Transcription activator-like (TAL) effectors specifically bind to double stranded (ds) DNA through a central domain of tandem repeats. Each TAL effector (TALE) repeat comprises 33–35 amino acids and recognizes one specific DNA base through a highly variable residue at a fixed position in the repeat. The crystal structures of TAL effector (TALE) proteins bound to their respective target DNAs have revealed that the residue at position 13 is the only one directly involved in DNA base recognition, whereas the 12th residue stabilizes the proper loop conformation. dHax3, an engineered TALE protein, proved to be a useful scaffold for structural characterizations. We then present fifteen crystal structures of engineered dHax3 variants in complex with target DNA molecules, which elucidate the structural basis for the recognition of bases adenine (A) and guanine (G) by reported or uncharacterized TALE codes.

When the natural TALE codes were discovered, no code was found highly specific for base G. In light of the structures of the DNA-binding zinc finger proteins where positive charged amino acids such as Arg, His, Lys play a critical role in the coordination of base G, we made a dHax3 variant with an Arg34, His34, Lys34 in the 7th repeat. We then attempted to co-crystallize these proteins with a modified dHax3 box element whose 7th base is changed from A to G. Four complex structures were determined at high resolutions.

>[2x]MQWSGARALEALLTVAGELRGPPLQLDTGQLLKIAKRGGVTAVEAVHAWRNALTGAPLNLTPEQVVAIASHDGGKQALETVQRLLPVLCQAHGLTPQQVVAIASHDGGKQALETVQRLLPVLCQAHGLTPEQVVAIASHDGGKQALETVQALLPVLCQAHGLTPEQVVAIASNGGGKQALETVQRLLPVLCQAHGLTPQQVVAIASNGGGKQALETVQRLLPVLCQAHGLTPQQVVAIASNGGGKQALETVQRLLPVLCQAHGLTPQQVVAIASNKGGKQALETVQRLLPVLCQAHGLTPQQVVAIASNGGGKQALETVQRLLPVLCQAHGLTPQQVVAIASHDGGKQALETVQRLLPVLCQAHGLTPEQVVAIASNGGGKQALETVQRLLPVLCQAHGLTPEQVVAIASHDGGKQALETVQRLLPVLCQAHGLTPQQVVAIASNGGGRPALESIVAQLSRPDPALAALTNDHLVALACLGGRPALDAVKKLEHHHHHH>VLSYHDSIKDAKKSVVNISTSKTITRANRPSPLDDFFNDPYFKQFFDFDFPQRKGKNDKEVVSSLGSGVIISKDGYIVTNNHVVDDADTITVNLPGSDIEYKAKLIGKDPKTDLAVIKIEANNLSAITFTNSDDLMEGDVVFALGNPFGVGFSVTSGIISALNKDNIGLNQYENFIQTDASINPGNSGGALVDSRGYLVGINSAILSRGGGNNGIGFAIPSNMVKDIAKKLIEKGKIDRGFLGVTILALQGDTKKAYKNQEGALITDVQKGSSADEAGLKRGDLVTKVNNKVIKSPI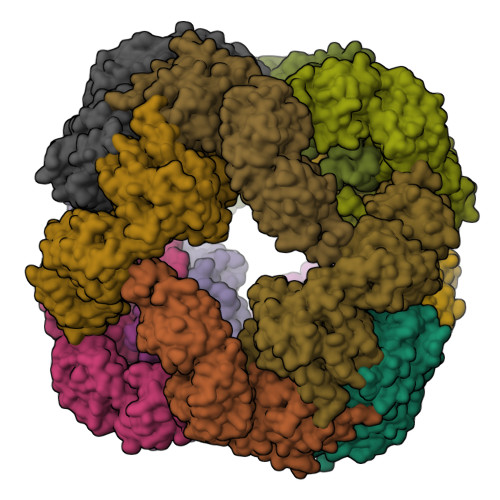DLKNYIGTLEIGQKISLSYERDGENKQASFILKGEKENPKGVQSDLIDGLSLRNLDPRLKDRLQIPKDVNGVLVDSVKEKSKGKNSGFQEGDIIIGVGQSEIKNLKDLEQALKQVNKKEFTKVWVYRNGFATLLVLK[12x]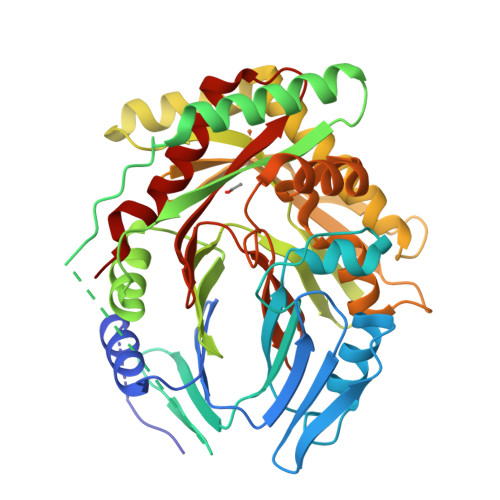>[2x]MKISEFLHLALPEEQWLPTISGVLRQFAEEECYVYERQPCWYLGKGCQARLHINADGTQATFIDDAGEQKWAVDSIADCARRFMAHPQVKGRRVYGQVGFNFAAHARGIAFNAGEWPLLTLTVPREELIFEKGNVTVYADSADGCRRLCEWVKEASTTTQNAPLAVDTALNGEAYKQQVARAVAEIRRGEYVKVIVSRAIPLPSRIDMPATLLYGRQANTPVRSFMFRQEGREALGFSPELVMSVTGNKVVTEPLAGTRDRMGNPEHNKAKEAELLHDSKEVLEHILSVKEAIAELEAVCLPGSVVVEDLMSVRQRGSVQHLGSGVSGQLAENKDAWDAFTVLFPSITASGIPKNAALNAIMQIEKTPRELYSGAILLLDDTRFDAALVLRSVFQDSQRCWIQAGAGIIAQSTPERELTETREKLASIAPYLMV>MGHHHHHHHHHHHHSSGHIDDDDKHMLEMIQSHPLLAAPLAVGDTIGFFSSSAPATVTAKNRFFRGVEFLQRKGFKLV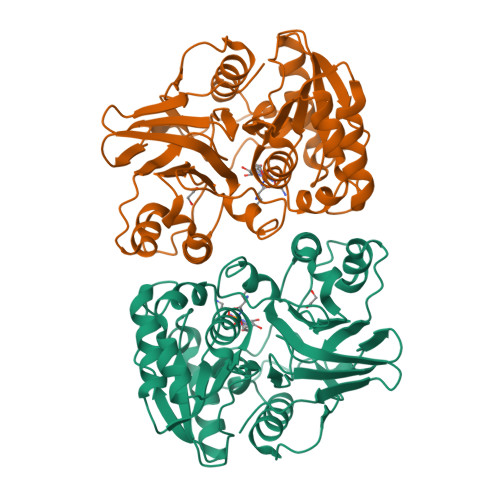SGKLTGKTDFYRSGTIKERAQEFNELVYNPDITCIMSTIGGDNSNSLLPFLDYDAIIANPKIIIGYADTTALLAGIYAKTGLITFYGPALIPSFGEHPPLVDITYESFIKILTRKQSGIYTYTLPEKWSDESINWNENKILRPKKLYKNNCAFYGSGKVEGRVIGGNLNTLTGIWGSEWMPEIRNGDILFIEDSRKSIATVERLFSMLKLNRVFDKVSAIILGKHELFDCAGSKRRPYEVLTEVLDGKQIPVLDGFDCSHTHPMLTLPLGVKLAIDFDNKNISITEQYLSTEK[2x]>[2x]SMSLLDAHIPQLIASEANFGAKAALMRSTIAQAEQAAMSSQAFHMGEASAAFQAAHARFVEVSAKVNALLDIAQLNIGDAASSYVAQDAAAASTYTGI;>MSQIMY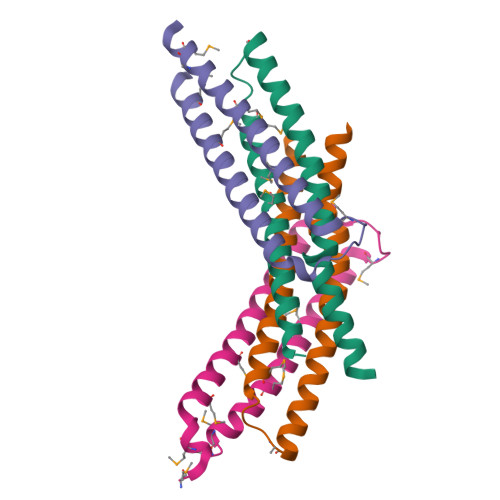NYPAMLAHAAEMNTYSGALHAVGADIAAEQHALASAWQGDTGMTYQAWQAQWNQAMEELVRAYRAMATTHEQNTMAMSARDQAEGAKWGTHHHHHH[2x]Here we report on the structural and biochemical characterization of PET46 (RLI42440.1), an archaeal promiscuous feruloyl esterase exhibiting degradation activity on semi-crystalline PET powder comparable to IsPETase and LCC (wildtypes), and higher activity on bis-, and mono-(2-hydroxyethyl) terephthalate (BHET and MHET). The enzyme, found by a sequence-based metagenome search, is derived from a non-cultivated, deep-sea Candidatus Bathyarchaeota archaeon. Biochemical characterization demonstrated that PET46 is a promiscuous, heat-adapted hydrolase. It shares the core alpha/beta-hydrolase fold with bacterial PETases, but contains a unique lid common in feruloyl esterases, which is involved in substrate binding.

The best PET46 crystal grew in space group P 61 2 2 and diffracted to a resolution of 1.71 Å. We could unambiguously model the protein chain in the electron density between residues 1–269. One monomer is present in the asymmetric unit (ASU), which shares the common fold of the α/β-hydrolase superfamily, with the core of the enzyme being composed of eight β-strands connected by seven α-helixes. In addition, a lid domain composed of three α-helixes and two anti-parallel β-strands is present (Leu141-Val186). The active site is composed of the catalytic triad Asp206, His238, and Ser115, as inferred from structure homology to other α/β-hydrolases. A phosphate ion and two ethylene glycol molecules were present near the active site, likely coming from the protein buffer, crystallization solution, and cryoprotectant. The bacterial and the archaeal enzymes present the typical residues of Ser-hydrolases at the catalytically active positions (Ser, His and Asp), but PET46 lacks a Trp associated with PET binding and formation of the aromatic clamp in the IsPETase and LCC. Nevertheless, the lack of an equivalent to Trp185 in IsPETase or Trp190 in LCC suggests that PET46 adopts a distinct substrate-binding pattern, probably involving the lid domain in the formation of the aromatic clamp. The largest difference is the medium-sized lid comprising 45 aa in PET46 (Leu141-Val186). Further structural differences around the active site are found in the enlarged loop between β4 and α3 (Loop 1; Asp68-Glu78; deep blue in Fig. 2a), which folds back to the outside, and the shorter loop between β10 and α10 containing the catalytic His (Loop 2; Arg234-Arg242; magenta in Fig. 2a). Note that the lid of PET46 has potentially adopted a non-optimal conformation/orientation for substrate binding.

> MIKPVTFMSEGEQIIGVLHVPDDLRGDKRAPAIAMFHGFTGNKSEAHRLFVHVARSLCNDGFVVLRFDFRGSGDSDGEFEDMTVPGEVCDASRSIDFLSELNFVDSERIGVLGLSMGGRVAAILASKDRRIKFVILYSAALTPLRRKFLEGLEKESIRRLEMGEAVHVGNGWYLKKGFFETVDSIVPLDVLDRIRVPVLIIHGDSDSVIPLDGALKGYEIIRDLNDKNELYIVRGGDHVFTRREHTIEVIERTLDWLRSLNLVDKLAAALEHHHHHH> MDNLLRHLKISKEQITPVVLVVGDPGRVDKIKVVCDSYVDLAYNREYKSVECHYKGQKFLCVSHGVGSAGCAVCFEELCQNGAKVIIRAGSCGSLQPDLIKRGDICICNAAVREDRVSHLLIHGDFPAVGDFDVYDTLNKCAQELNVPVFNGISVSSDMYYPNKIIPSRLEDYSKANAAVVEMELATLMVIGTLRKVKTGGILIVDGCPFKWDEGDF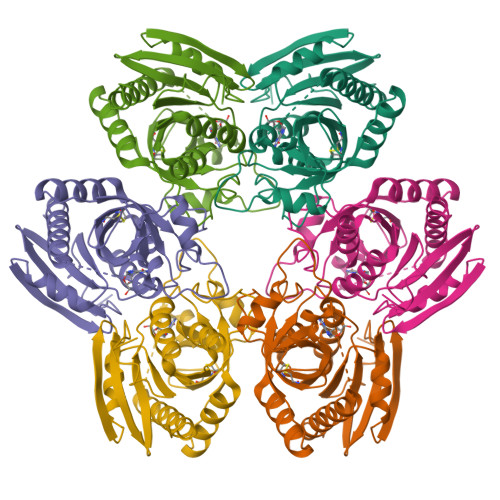DNNLVPHQLENMIKIALGACAKLATKYALEHHHHHH> MEQIQMVKVLEKCQVTPPSDTTDVELSLPVTFFDIPWLHLNKMQSLLFYDFPYPRTHFLDTVIPNLKAS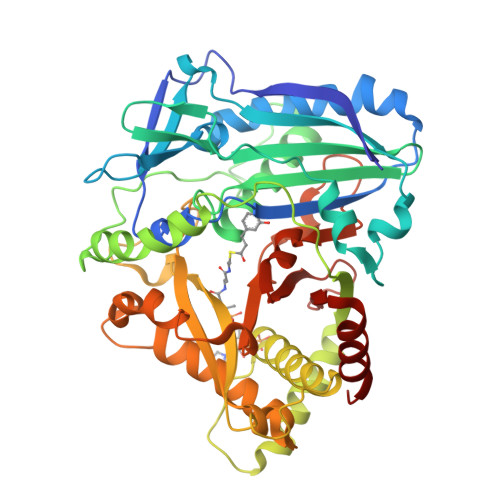LSLTLKHYVPLSGNLLMPIKSGEMPKFQYSRDEGDSITLIVAESDQDFDYLKGHQLVDSNDLHGLFYVMPRVIRTMQDYKVIPLVAVQVTVFPNRGIAVALTAHASIADAKSFVMFINAWAYINKFGKDADLLSANLLPSFDRSIIKDLYGLEETFWNEMQDVLEMFSRFGSKPPRFNKVRATYVLSLAEIQKLKNKVLNLRGSEPTIRVTTFTMTCGYVWTCMVKSKDDVVSEESSNDENELEYFSFTADCRGLLTPPCPPNYFGNCLASCVAKATHKELVGDKGLLVAVAAIGEAIEKRLHNEKGVLADAKTWLSESNGIPSKRFLGITGSPKFDSYGVDFGWGKPAKFDITSVDYAELIYVIQSRDFEKGVEIGVSLPKIHMDAFAKIFEEGF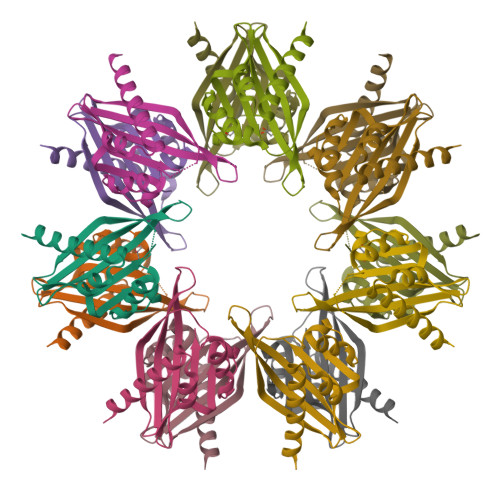>GPHSEDEEGQDVTAKVREQEIIRLTQKLITSITTGDYDTYSKLVDPHVTCFEPFSNGNLVEGLEFHKFYFDNTLSKRSVPINTTILSPHVHVLGEDAACICYMRLTQSVNSSGEAKTLQQEETRVWQKKGGNWINVHFHISGKMS[7x]> MKRQGKRPSKNLKARCSRKALHVNFKDMGWDDWIIAPLEYEAFHCEGLCEFPLRSHLEPTNH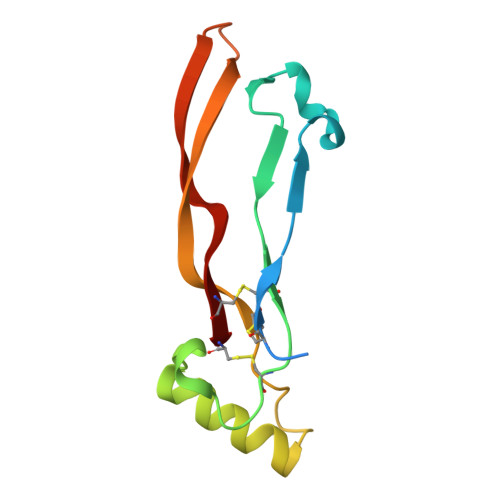AVIQTLMNSMDPESTPPTCCVPTRLSPISILFIDSANNVVYKQYEDMVVESCGCR> MEQQPLTLTAATTRAQELRKQLNQYSHEYYVKDQPSVEDYVYDRLYKELVDIETEFPDLITPDSPTQRVGGKVLSGFEKAPHDIPMYSLNDGFSKED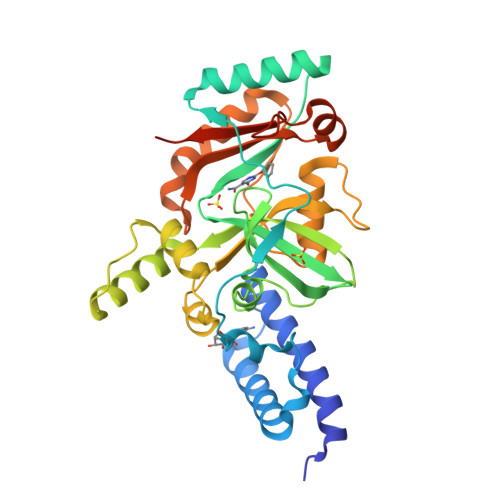IFAFDERVRKAIGKPVAYCCELKIDGLAISLRYENGVFVRGATRGDGTVGENITENLRTVRSVPMRLTEPISVEVRGECYMPKQSFVALNEEREENGQDIFANPRNAAAGSLRQLDTKIVAKRNLNTFLYTVADFGPMKAKTQFEALEELSAIGFRTNPERQLCQSIDEVWAYIEEYHEKRSTLPYEIDGIVIKVNEFALQDELGFTVKAPRWAIAYKFPPEEAETLEHHHHHH> MESKLNLDFNLVEKARAKAKAIAIDTQEFIEKHTTVTVERAVCRLLGIDGVDTDEVPLPNIVVDHIKENNGLNLGAAMYIANAVLNTGKTPQEIAQAISAGELDLTKLPMKDLFEVKTKALSMAKE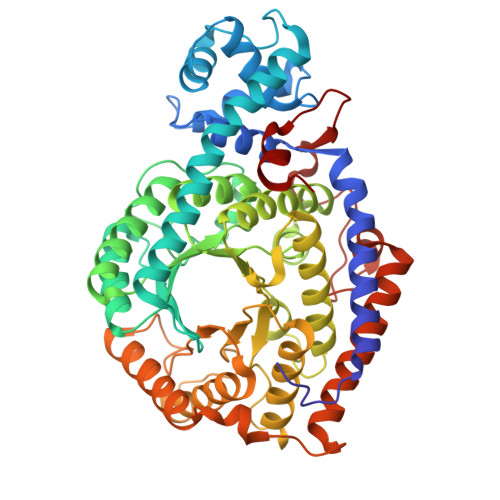TVEKIKNNRSIRESRFEEYGDKSGPLLYVIVATGNIYEDITQAVAAAKQGADVIAVIRTTGQSLLDYVPYGATTEGFGGTYATQENFRLMREALDKVGAEVGKYIRLCNYCSGLCMPEIAAMGAIERLDVMLNDALYGILFRDINMQRTMIDQNFSRIINGFAGVIINTGEDNYLTTADAFEEAHTVLASQFINEQFALLAGLPEEQMGLGHAFEMDPELKNGFLYELSQAQMAREIFPKAPLKYMPPTKFMTGNIFKGHIQDALFNMVTIMTNQRIHLLGMLTEALHTPFMSDRALSIENAQYIFNNMESISEEIQFKEDGLIQKRAGFVLEKANELLEEIEQLGLFDTLEKGIFGGVKRPKDGGKGLNGVVSKDENYYNPFVELMLNK> TSVN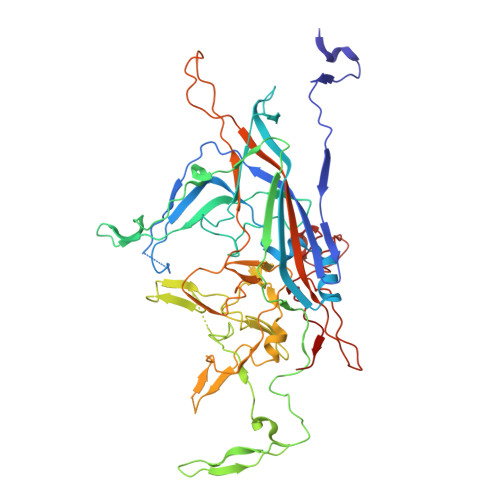SAEASTGAGGGGSNPVKSMWSEGATFSANSVTCTFSRQFLIPYDPEHHYKVFSPAASSCHNASGKEAKVCTISPIMGYSTPWRYLDFNALNLFFSPLEFQHLIENYGSIAPDALTVTISEIAVKDVTDKTGGGVQVTDSTTGRLCMLVDHEYKYPYVLGQGQDTLAPELPIWVYFPPQYAYLTVGDVNTQGISGDSKKLASEESAFYVLEHSSFQLLGTGGTATMSYKFPPVPPENLEGCSQHFYEMYNPLYGSRLGVPDTLGGDPKFRSLTHEDHAIQPQNFMPGPLVNSVSTKEGDSSNTGAGKALTGLSTGTSQNTRISLRPGPVSQPYHHWDTDKYVTGINAISHGQTTYGNAEDKEYQQGVGRFPNEKEQLKQLQGLNMHTYFPNKGTQQYTDQIERPLMVGSVWNRRALHYESQLWSKIPNLDDSFKTQFAALGGWGLHQPPPQIFLKILPQSGPIGGIKSMGITTLVQYAVGIMTVTMTFKLGPRKATGRWNPQPGVYPPHAAGHLPYVLYDPTATDAKQHHRHGYEKPEELWTAKSRVHPL>[4x]MHVRDTKLTVDDITGVVGIIPTPSIPTADQPGTAFSVDLDEAATLADAMVRGGVDVLMTTGTFGECASLTWDELQSFVATVVDAVAGRIPVFAGATTLNTRDTIARGRRLGELGADGLFVGRPMWLPLDDAGIVRFYRDVAEAVPNMALVVYDNPGAFKGKIGTPAYEALSQIPQVVAAKHLGLLSGSAFLSDLRAV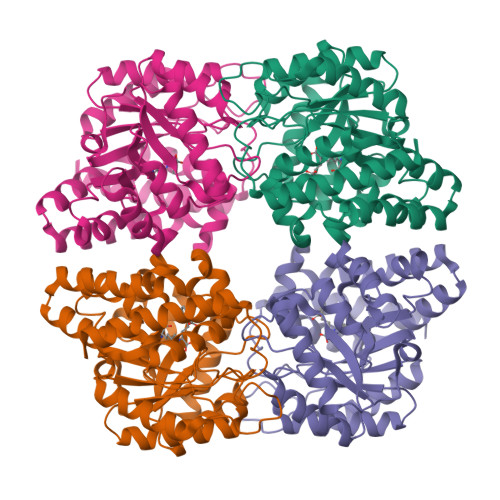SGRVRLLPLETDWYYFARLFPEEVTACWSGNVACGPAPVTHLRDLIRARRWDDCQALTDELEGALETLYPGGNFAEFLKYSIQIDNAQFQAAGFMRTGPTRPPYTEVPESYLAGGREAGKNWAALQQRYASLAVSNH>[13x]MAEKRTGLAEDGAKSVYERLKNDRAPYETRAQNCAQYTIPSLFPKDSDNASTDYQTPWQAVGARGLNNLASKLMLALFPMQTWMRLTISEYEAKQLLSDPDGLAKVDEGLSMVERIIMNYIESNSYRVTLFEALKQLVVAGNVLLYLPEPEGSNYNPMKLYRLSSYVVQRDAFGNVLQMVTRDQIAFGALPEDIRKAVEGQGGEKKADETIDVYTHIYL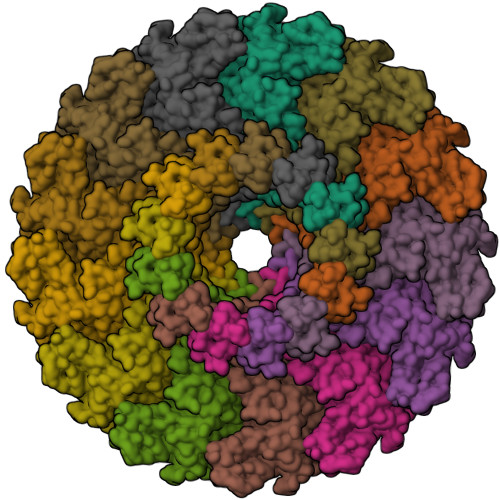DEDSGEYLRYEEVEGMEVQGSDGTYPKEACPYIPIRMVRLDGESYGRSYIEEYLGDLRSLENLQEAIVKMSMISSKVIGLVNPAGITQPRRLTKAQTGDFVTGRPEDISFLQLEKQADFTVAKAVSDAIEARLSFAFMLNSAVQRTGERVTAEEIRYVASELEDTLGGVYSILSQELQLPLVRVLLKQLQATQQIPELPKEAVEPTISTGLEAIGRGQDLDKLERCVTAWAALAPMRDDPDINLAMIKLRIANAIGIDTSGILLTEEQKQQKMAQQSMQMGMDNGAAALAQGMAAQATASPEAMAAAADSVGLQPGI8-hydroxyquinoline 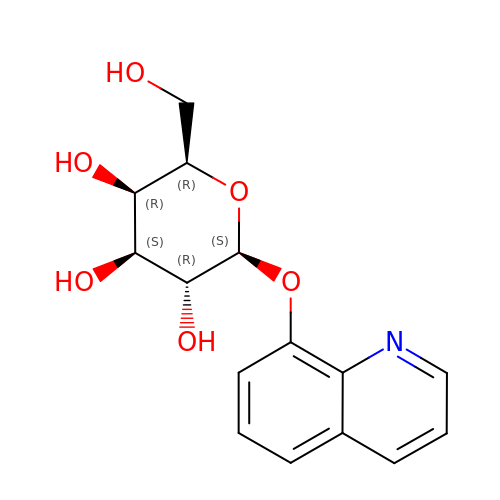beta-galactopyranoside | C15 H17 N O6 | BWMXDESAZVPVGR-BGNCJLHMSA-N>[2x]SRLN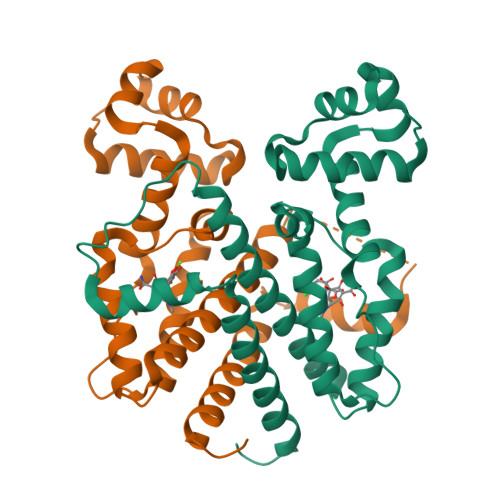RESVIDAALELLNETGIDGLTTRKLAQKLGIEQPTLYWHVKNKRALLDALAVEILARHHDYSLPAAGESWQSFLRNNAMSFRRALLRYRDGAKVHLGTRPDEKQYDTVETQLRFMTENGFSLRDGLYAISAVSHFTLGAVLEQQEHTAALTDRPAAPDENLPPLLREALQIMDSDDGEQAFLHGLESLIRGFEVQLTALLQIV> GIYGIGLDITEL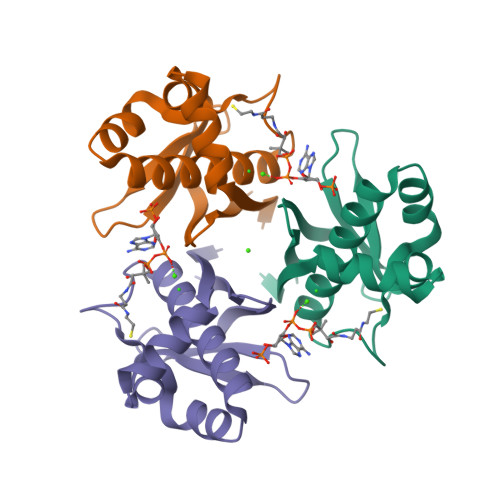KRIASMAGRQKRFAERILTRSELDQYYELSEKRKNEFLAGRFAAKEAFSKAFGTGIGRQLSFQDIEIRKDQNGKPYIICTKLSPAAVHVSITHTKEYAAAQVVIERLSS>MAHHHHHHMAASPEAKFTEEKILWVKHHTPKLITFAISRPESYRFKAGQFSRLGFYEGKGFIWRAYSVVSAEYADTLEYFAVLIQDGPMSALFAKMQQGDTILLDKN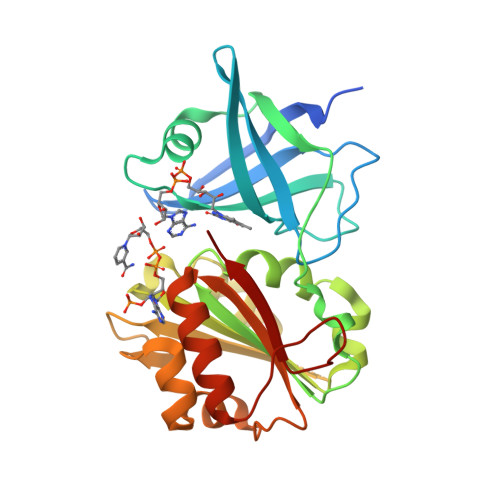ATGFLLPERFPDGKDLVMLCTGSGIAPFLSILEQPEIRQRFDTVNLIHSVSFPEELIFNDRLAALSEHPLVGEYGHSFRFVPVTTRAANPSGLSGKRIPELLKNNSIEQALHTKLTPESTRFMICGNPEMVKDTFQTLLDMGYAMHRNRIPGQIMMENGF[3x]>[2x]SNAGFQQSHYFVALYRFKALEKDDLDFRPGEKITVIDDSNEEWWRGKIGEKVGFFPPNFIIRVRAGERVHRVTRSFVGNREIGQITLNKDQIVVQKGDEAGGYVKVYTGR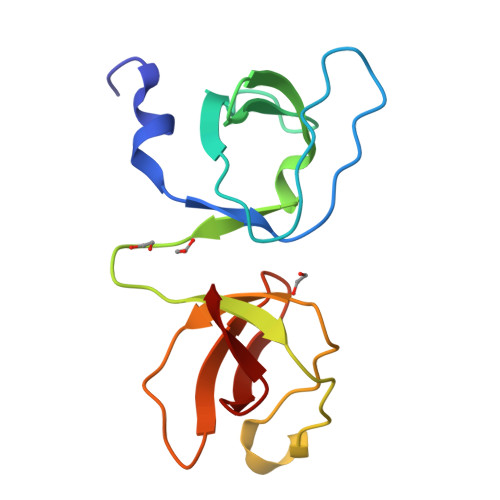KVGLFPTDFLEEI> SHMLRPVETPTREIKKLDGLWAFSLDRENCGIDQRWWESALQESRAIAVPGSFNDQFADADIRNYAGNVWYQREVFIPKGWAGQRIVLRFDAVTHYGKVWVNNQEVMEHQGGYTPFEADVTPYVIAGKSVRITVCVNNELNWQTIPPGMVITDENGKKKQSYFHDFFNYAGIHRSVMLYTTPNTWVDDITVVTHVAQDCNHASVDWQVVANGDVSVELRDADQQVVATGQGTSGTLQVVNPHLWQPGEGYLYELCV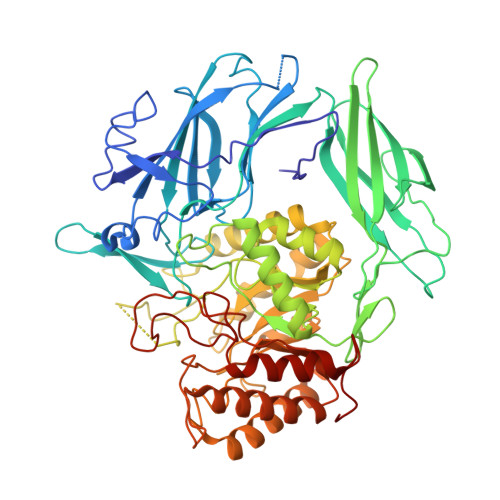TAKSQTECDIYPLRVGIRSVAVKGEQFLINHKPFYFTGFGRHEDADLRGKGFDNVLMVHDHALMDWIGANSYRTSHYPYAEEMLDWADEHGIVVIDETAAVGFNLSLGIGFEAGNKPKELYSEEAVNGETQQAHLQAIKELIARDKNHPSVVMWSIANEPDTRPQGAREYFAPLAEATRKLDPTRPITCVNVMFCDAHTDTISDLFDVLCLNRYYGWYVQSGDLETAEKVLEKELLAWQEKLHQPIIITEYGVDTLAGLHSMYTDMWSEEYQCAWLDMYHRVFDRVSAVVGEQVWNFADFATSQGILRVGGNKKGIFTRDRKPKSAAFLLQKRWTGMNFGEKPQQGGKQ>[24x]GIPGMLPWPKVDFSKFGEIEEVELGRIQKISGANLSRNWVMIPHVTHFDKTDITELEAFRKQQNEEAAKRKLDVKITPVVFI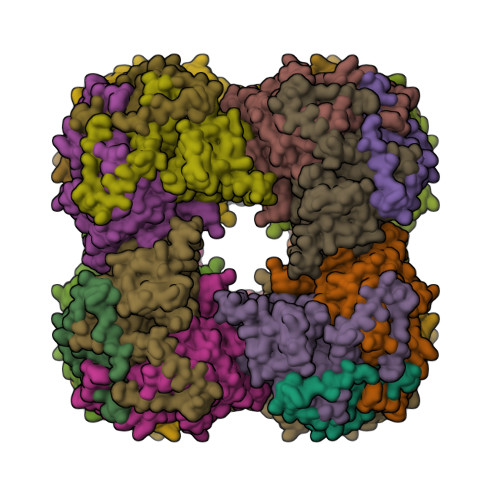MKAVAAALEQMPRFNSSLSEDGQRLTLKKYINIGVAVDTPNGLVVPVFKDVNKKGIIELSRELMTISKKARDGKLTAGEMQGGCFTISSIGGLGTTHFAPIVNAPEVAILGVSKSAMEPVWNGKEFVPRLMLPISLSFDHRVIDGADGARFITIINNTLSDIRRLVM>MRYRLAWLLHPALPSTFRSVLGARLPPPERLCGFQKKTYSKMNNPAIKRIGNHITKSPEDKREY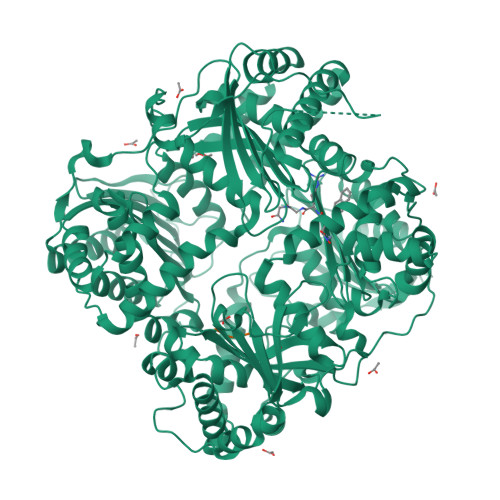RGLELANGIKVLLISDPTTDKSSAALDVHIGSLSDPPNIAGLSHFLQHMLFLGTKKYPKENEYSQFLSEHAGSSNAFTSGEHTNYYFDVSHEHLEGALDRFAQFFLSPLFDESAKDREVNAVDSEHEKNVMNDAWRLFQLEKATGNPKHPFSKFGTGNKYTLETRPNQEGIDVRQELLKFHSAYYSSNLMAVVVLGRESLDDLTNLVVKLFSEVENKNVPLPEFPEHPFQEEHLKQLYKIVPIKDIRNLYVTFPIPDLQKYYKSNPGHYLGHLIGHEGPGSLLSELKSKGWVNTLVGGQKEGARGFMFFIINVDLTEEGLLHVEDIILHMFQYIQKLRAEGPQEWVFQELKDLNAVAFRFKDKERPRGYTSKIAGILHYYPLEEVLTAEYLLEEFRPDLIEMVLDKLRPENVRVAIVSKSFEGKTDRTEEWYGTQYKQEAIPDEVIKKWQNADLNGKFKLPTKNEFIPTNFEILPLEKEATPYPALIKDTAMSKLWFKQDDKFFLPKANLNFEFFSPFAYVDPLHSNMAYLYLELLKDSLNEYAYAAELAGLSYDLQNTIYGMYLSVKGYNDKQPILLKKIIEKMATFEIDEKRFEIIKEAYMRSLNNFRAEQPHQHAMYYLRLLMTEVAWTKDELKEALDDVTLPRLKAFIPQLLSRLHIEALLHGNITKQAALGIMQMVEDTLIEHAHTKPLLPSQLVRYREVQLPDRGWFVYQQRNEVHNNSGIEIYYQTDMQSTSENMFLELFAQIISEPAFNTLRTKEQLGYIVFSGPRRANGIQGLRFIIQSEKPPHYLESRVEAFLITMEKSIEDMTEEAFQKHIQALAIRRLDKPKKLSAESAKYWGEIISQQYNFDRDNTEVAYLKTLTKEDIIKFYKEMLAVDAPRRHKVSVHVLAREMDSNPVVGEFPAQNDINLSQAPALPQPEVIQNMTEFKRGLPLFPLVKPHINFMAAKL[2x];>AAA[2x]> MYYGISQFSEAYNKILRNSSSASSCQLVIFVSCLNIDALCATKMLSLLFKKQLVQSQIVPIFGYSELRRHYSQLDDNINSLLLVGFGGVIDLEAFLEIDPQEYVIDTDEKSGEQSFRRDIYVLDAHRPWNLDNIFGSQIIQCFDDGTVDDTLGEEKEAYYKLLELDEESGDDELSGDENDNNGGDDEATDADEVTDEDEEDEDETISNKRGNSSIGPNDLSKRKQRKKQIHEYEGVLEEYYSQGTTVVNSISAQIYSLLSAIGETNLSNLWLNILGTTSLDIAYAQVYNRLYPLLQDEVKRLTPSSRNSVK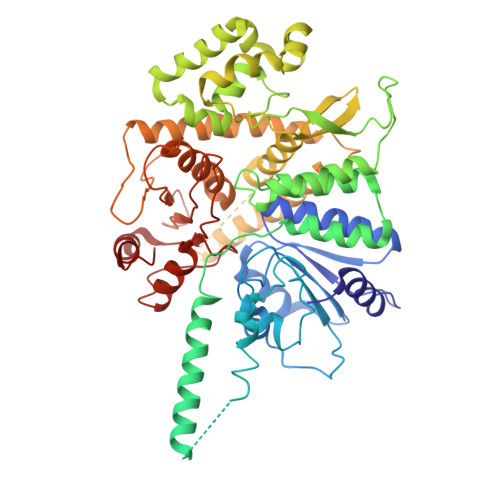TPDTLTLNIQPDYYLFLLRHSSLYDSFYYSNYVNAKLSLWNENGKKRLHKMFARMGIPLSTAQETWLYMDHSIKRELGIIFDKNLDRYGLQDIIRDGFVRTLGYRGSISASEFVEALTALLEVGNSTDKDSVKINNDNNDDTDGEEEEDNSAQKLTNLRKRWVSNFWLSWDALDDRKVELLNRGIQLAQDLQRAIFNTGVAILEKKLIKHLRIYRLCVLQDGPDLDLYRNPLTLLRLGNTLIECCAESEDKQLLPMVLASIDENTDTYLVAGLTPRYPRGLDTIHTKKPILNNFSMAFQQITAETDAKVRIDNFESSIIEIRREDLSPFLEKLTLSGLL>MNKILLVDDDRELTSLLKELLEMEGFNVIVAHDGEQALDLLDDSIDLLLLDVMMPKKNGIDTLKALRQTHQTPVIMLTARGSELDRVLGLELGADDYLPKPFNDRELVARIRAILRRSHWSEQKLAAALEHHH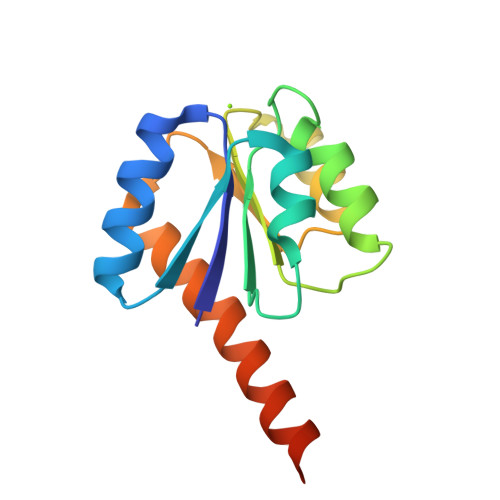HHH[3x]>MFKRFSKKKEAPED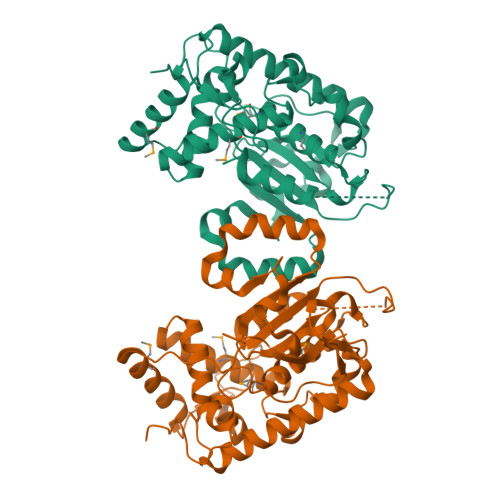PKNLINIDKPIKELPASIAIPKEKPLTGEQQKMYDEVLKHFSNPDLKVYTSEKNKSEDDLKPLEEEEKAWLTRECFLRYLRATKWVLKDCIDRITMTLAWRREFGISHLGEEHGDKITADLVAVENESGKQVILGYENDARPILYLKPGRQNTKTSHRQVQHLVFMLERVIDFMPAGQDSLALLIDFKDYPDVPKVPGNSKIPPIGVGKEVLHILQTHYPERLGKALLTNIPWLAWTFLKLIHPFIDPLTREKLVFDEPFVKYVPKNELDSLYGGDLKFKYNHDVYWPALVETAREKRDHYFKRFQSFGGIVGLSEVDLRGTHEKLLYPVKSESSTV[2x]>[7x]MADISRADALALLATQELDSIIKPETSGSAALAAFRSIRMSAGTVSMPVLAALPTAGWVTDDTSGAATGTKPTSKVSWTGKNLVAEEIAVIVPVHENTIADSRFDIWGEVRPLVSQEFGRVLDEAVFFGVNKP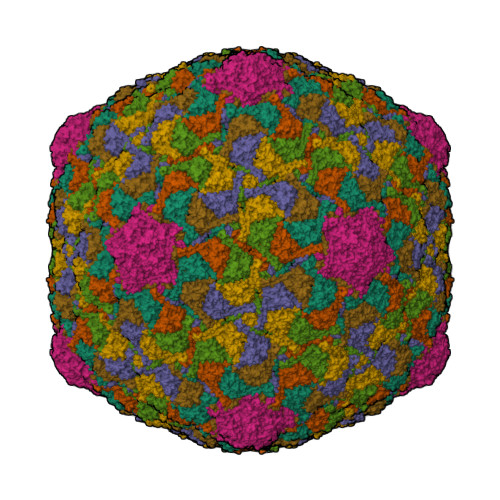ATWLDPALVPGAIAAGNTIADGTGIDLADDINEAFGFVEDDEFDVNVAFTGRFLRRRLRGLRDADNAPIYLDGVRSDNRTAEIYGQDLMYVGNRSWDRDEAVLLAGDRSKVLLGIREDVQVKLLTEATIGGINLAEKDMVALRFKFRVAYSTAFSTAGGEVTDYPFAVITPDVTP> GPGYQDPLSIDSKIQYITYTNLKAAVEKFHAKAGAAMVIDVQTGEVLSLVNYPGRNRVLTDVFEPGSIMKPFTVSLALDLHRVTPNTLVETGNGHFVLDGAPITDDSGFGTLTVGGVIQKSSNIGATKIAMTMKPEEMWNMYTGIGLGQAPKVGFPGAAAGRLRPWKNWRRIEQATMSYGYGLSVSLFQLARAYTAIAHDGELMPVTIFKTNDAQPPTGPRVFSPTTAREVRTMLESVVSPQGTSPNAAVPGYRVGGKSGTAYKQVGRGYDHKKYRASFVGMAPMPNPRIVVAVSVDEPTTGGHFGGQVSGPVFSAIVGDTLRALNVPPNMPVKQ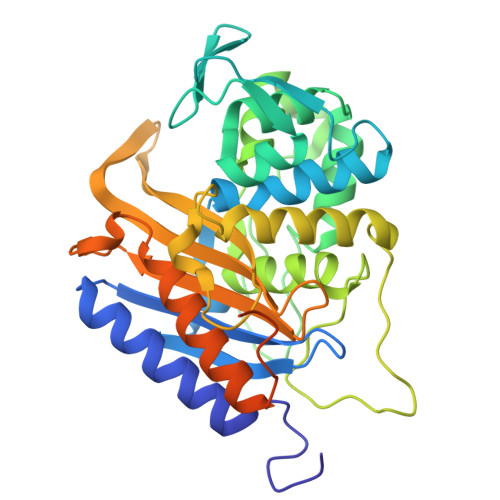LVVSDDATNAAAAQKLAANAPAKRLIVSSTTHNRPGVVR> MAESKPTPQSTFTGPIVVDPITRIEGHLRIMVEVENGKVKDAWSSSQLFRGLEIILKGRDPRDAQHFTQRACGVCTYVHALASSRCV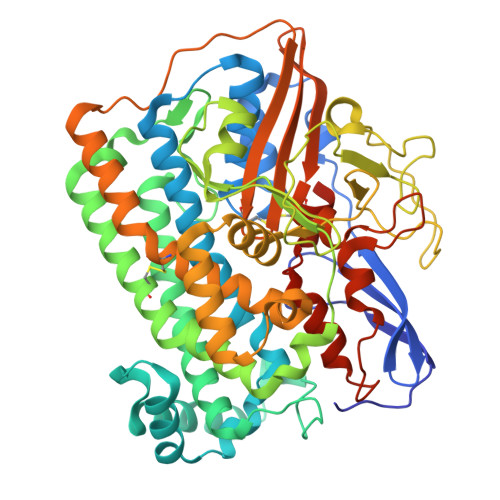DDAVKVSIPANARMMRNLVMASQYLHDHLVHFYHLHALDWVDVTAALKADPNKAAKLAASIDTARTGNSEKALKAVQDKLKAFVESGQLGIFTNAYFLGGHKAYYLPPEVNLIATAHYLEALHMQVKAASAMAILGGKNPHTQFTVVGGCSNYQGLTKDPLANYLALSKEVCQFVNECYIPDLLAVAGFYKDWGGIGGTSNYLAFGEFATDDSSPEKHLATSQFPSGVITGRDLGKVDNVDLGAIYEDVKYSWYAPGGDGKHPYDGVTDPKYTKLDDKDHYSWMKAPRYKGKAMEVGPLARTFIAYAKGQPDFKKVVDMVLGKLSVPATALHSTLGRTAARGIETAIVCANMEKWIKEMADSGAKDNTLCAKWEMPEESKGVGLADAPRGSLSHWIRIKGKKIDNFQLVVPSTWNLGPRGPQGDKSPVEEALIGTPIADPKRPVEILRTVHAFDPCIACGVHVIEPETNEILKFKVC> GAMGSKPDTHRADERRFLDERGSSGPLAPNGLNPATIMEKAVRERIVESYFWKEQCFGVNEADIVDRVVEHVRFVGGVTGVTQKPSPFLCLAFKLLQLAPGDDILKEYLYFGGEKFKYLRALAAFYIRLTRPDKEVYT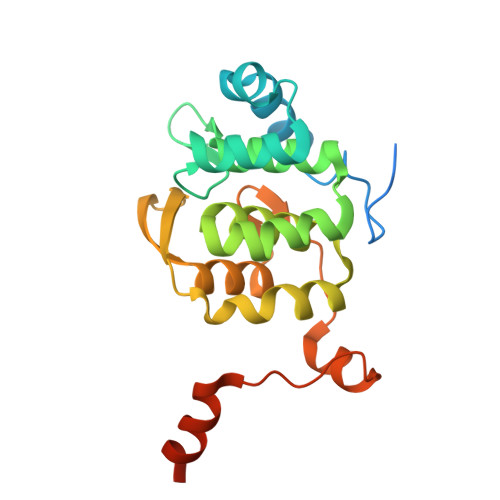LLEPFLEDRRKLRRKGKNGTSLTYMDEFIDDLLTKDRVCSTSLWKMRRRDILEDLDLLEPRVSPLGSLEDILEEEEQAAKNEDGE> GPHMRKSQQAEREYEKIKSQLEGLEESVRDRCKKEFTDLMIEMEDQTNDVHEAGIPTLDYKTYTDRVFFLPSKDGDKDVMITGKLDIPESRRPIVEQA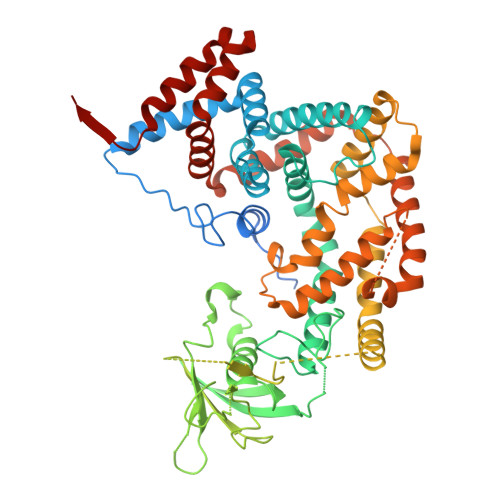LYQFSNLLNSKSFLINFIHTLENQREFSARAKVYFASLLTVALHGKLEYYTDIMRTLFLELMEQYVVAKNPKLMLRRSETVVERMLSNWMSICLYQYLKDSAGEPLYKLFKAIKHQVEKGPVDAVQKKAKYTLNDTGLLGDDVEYAPLTVSVIVQDEGIDAIPVKVLNCDTISQVKEKIIDQVYRTQPCSCWPKPDSVVLEWRPGSTAQILSDLDLTSQREGRWKRINTLMHYNVRDGATLILSKVGVSQQPEDSQQDLPGERHALLEEENRVWHLVRPTDEVDEGKSKRGSMKEKERTKAITEIYLTRLLSVKGTLQQFVDNFFQSVLAPGHAVPPAVKYFFDFLDEQAEKHDIRDEDTIHIWKTNSLPLRFWVNILKNPHFIFDVHVHEVVDASLSVIAQTFMDACTRTEHKLSRDSPSNKLLYAKEISTYKKMVEDYYKGIRQMVQVSDQDMNTHLAEISRAHTDSLNTLVALHQLYQYTQKYYDEIINALEEDPAAQKMQLAFRLQQIAAALENKVTDL> SNAFQNKANVCWAKSLVPILETAGIKLNDRQWSQIIQAFKEDKAYSPEVALNEICTRMYGVDLDSGLFSKPLVSVYYADNHWDNRPGGKMFGFNPEAASILERKYPFTKGKWNINKQICVTTRR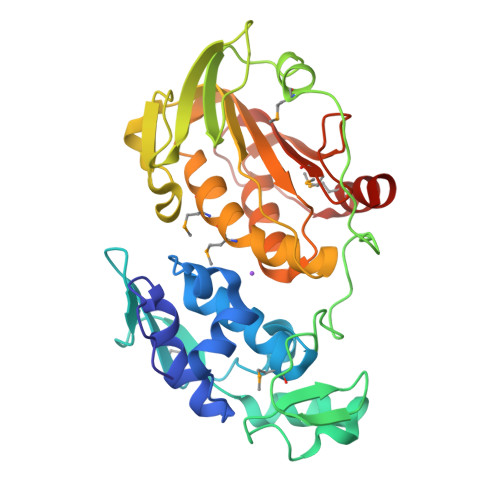IEDFNPTTNIIPVNRRLPHSLVAEHRPVKGERMEWLVNKINGHHVLLVSGYNLALPTKRVTWVAPLGVRGADYTYNLELGLPATLGRYDLVVINIHTPFRIHHYQQCVDHAMKLQMLGGDSLRLLKPGGSLLIRAYGYADRTSERVICVLGRKFRSSRALKPPCVTSNTEMFFLFSNFDNGRRNFTTHVMNNQLNAAFVG> GAMVETKCPNLDIVTSSGEFHCSGCVEHMPEFSYMYWLAKDMKSDEDTKFIEHLGDGINEDET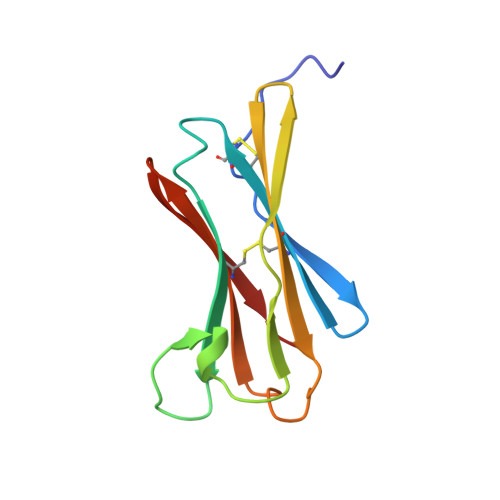VRTTDGGITTLRKVLHVTDTNKFAHYRFTCVLTTLDGVSKKNIWLK>MHLRHLFSSRLRGSLLLGSLLVVSSFSTQAAEEMLRKAVGKGAYEMAYSQQENALW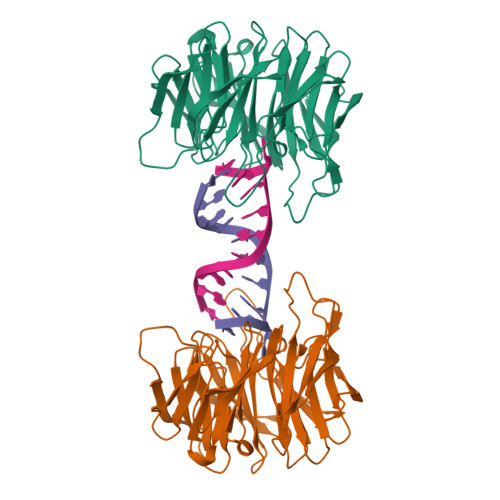LATSQSRKLDKGGVVYRLDPVTLEVTQAIHNDLKPFGATINNTTQTLWFGNTVNSAVTAIDAKTGEVKGRLVLDDRKRTEEVRPLQPRELVADDATNTVYISGIGKESVIWVVDGGNIKLKTAIQNTGKMSTGLALDSEGKRLYTTNADGELITIDTADNKILSRKKLLDDGKEHFFINISLDTARQRAFITDSKAAEVLVVDTRNGNILAKVAAPESLAVLFNPARNEAYVTHRQAGKVSVIDAKSYKVVKTFDTPTHPNSLALSADGKTLYVSVKQKSTKQQEATQPDDVIRIAL[4x]> GPMTSQKLVRLPGLIDVHVHLREPGGTHKEDFASGTAAALAGGITMVCAMPNTRPPIIDGPALALAQKLAEAGARCDFALFLGASSENAGTLGTVAGSAAGLKLYLNETLSELRLDSVVQWMEHFETWPSHLPIVAHAEQQTVAAVLMVAQLT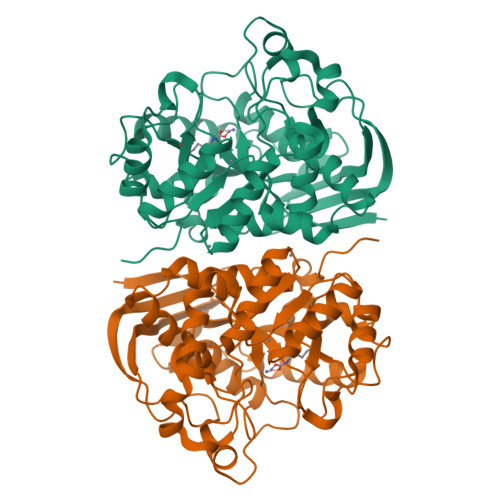QRSVHICHVARKEEILLIKAAKARGLPVTCEVAPHHLFLSHDDLERLGPGKGEVRPELGSRQDVEALWENMAVIDCFASDHAPHTLEEKCGSRPPPGFPGLETMLPLLLTAVSEGRLSLDDLLQRLHHNPRRIFHLPPQEDTYVEVDLEHEWTIPSHMPFSKAHWTPFEGQKVKGTVRRVVLRGEVAYIDGQVLVPPGYGQDVRKWPQGAVPQLPPSAPATSEMTTTPERPRRGIPGLPD> MLTRQARLLRRIPPPNAVLQSGLQRRHRSTDRYSNNIHTSSTQNAPAPVYDTPIREKGMTLEAKERVRAHVRKIQSSASTAAASPAVRPQPAQHFQAAPQPMPTNMPRFESDSQVKNGLDYSFIGLSGGQIFQEMMLRHDVKQVFGYPGGAILPVFDAIYNSPHFEFVLPRHEQGAGHMAEGYARVSGKPGVVLVTSGPGATNVITPMQDALSDGVPMVVF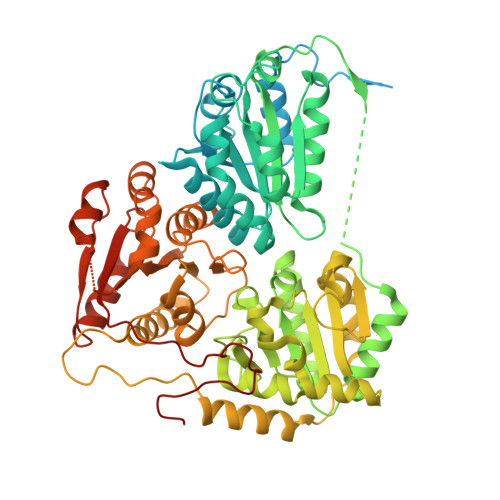CGQVATNLIGSDAFQEADVVGISRSCTKWNVMVKDIAELPRRINEAFKIATTGRPGPVLVDLPKDVTAAILRTPIPAKSVQPGHSPYLPSNPLNPSSQPSDPLPGDADLITEAAQMINKAKRPIIFAGNGVLSSPEGPKLLKELSDKGRIPVTTTLQGLGAFDERDEKSLHMIGMHGSAYANFAMQEADVLIALGVRFDDRVTGKVDTFAPAAKAAAAEGRGGIIHFEIQPKNINKIVEGQIPVLGDVVASLGELVPQIEAVDRSAWIGRCKATKERYPFTYTPSQEGQKLKPQEVVQELDRQAEALGKEKFVISTGVGQHQMWACQYYRWTEPRSWVSSGGLGTMGFGLPSAIGAKVAAPEKYVIDIDGDASFSMTAMELATASQYDIGVKVLLFNNEFQGMVEQWQDLFYENRYSRTRMTNPDFVKLSESMGAKGLRCTKLEDLPRMMKEFLEYDGKRPIVLECLVSSEHVYPMIPAGKALHEQLLHPLLRNGSE> MESIEQQLTELRTTLRHHEYLYHVMDAPEIPDAEYDRLMRELRELETKHPELITPDSPTQRVGAAPLAAFSQIRHEVPMLSLDNVFDEESFLAFNKRVQDRLKNNEKVTWCCELKLDGLAVSILYENGVLVSAATRGDGTTGEDITSNVRTIRAIPLKLHGENIPARLEVRGEVFLPQAGFEKINEDARRTGGKVFANPRNAAAGSLRQLDPRITAKRPLTFFCYGVGVLEGGELPDTHLGRLLQFKKWGLPVSDRVTLCESAEEVLAFYHKVEEDRPTLGFDIDGVVIKVNSLAQQEQLGFVARAPRWAVAFKFPAQEQMTFVRDVEFQVGRTGAITPVARLEPVHVAGVLVSNATLHNADEIERLGLRIGDKVVIRRAGDVIPQVVNVVLSERPEDTREVVFPTHCPVCGSD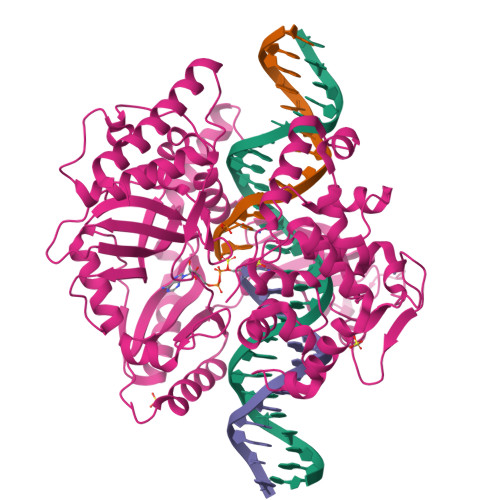VERVEGEAVARCTGGLICGAQRKESLKHFVSRRAMDVDGMGDKIIDQLVEKEYVHTPADLFKLTAGKLTGLERMGPKSAQNVVNALEKAKETTFARFLYALGIREVGEATAAGLAAYFGTLEALEAASIEELQKVPDVGIVVASHVHNFFAEESNRNVISELLAEGVHWPAPIVINAEEIDSPFAGKTVVLTGSLSQMSRDDAKARLVELGAKVAGSVSKKTDLVIAGEAAGSKLAKAQELGIEVIDEAEMLRLLGS> GSHMGSDELYRQSLEIISRYLREQATGAKDTKPMGRSGATSRKALETLRRVGDGVQRNHETAFQGMLRKLDIKNEDDVKSLSRVMIHVFSDGVTNWGRIVTLISFGAFVAKHLKTINQESCIEPLAESITDVLVRTKRDWLVKQRGWDGFVEFFHVE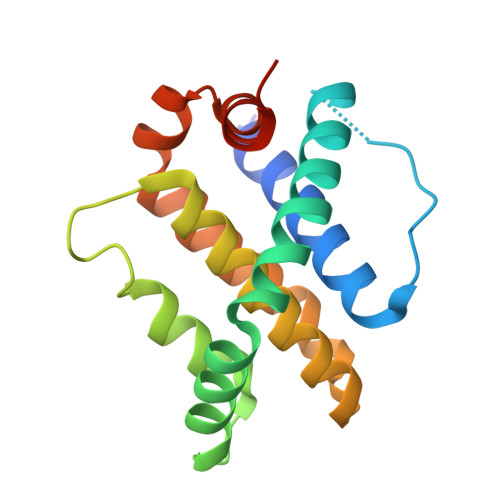DLEGG>[4x]EGPIDKLKTPEDVPNDPLPLISDFEWSTL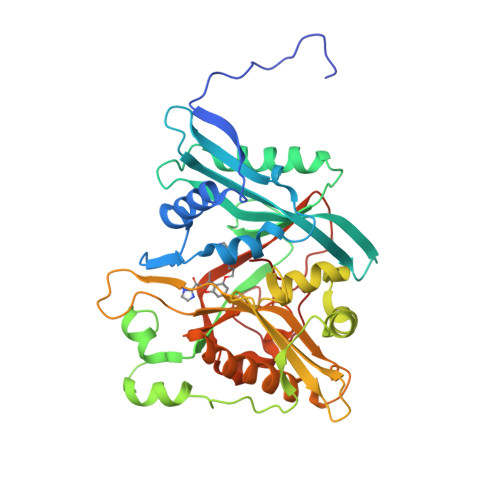DIDDNLQLDELYKLLYDNYVEDIDATFRFKYSHEFFQWALKPPGWRKDWHVGVRVKSTGKLVAFIAATPVTFKLNKSNKVIDSVEINFLCIHKKLRNKRLAPVLIKEITRRVNKQNIWQALYTGGSILPTPLTTCRYQHRPINWSKLHDVGFSHLPPNQTKSSMVASYTLPNNPKLKGLRPMTGKDVSTVLSLLYKYQERFDIVQLFTEEEFKHWMLGHDENSDSNVVKSYVVEDENGIITDYFSYYLLPFTVLDNAQHDELGIAYLFYYASDSFEKPNYKKRLNELITDALITSKKFGVDVFNCLTCQDNTYFLKDCKFGSGDGFLNYYLFNYRTFPMDGGIDKKTKEVVEDQTSGIGVVLL>MTKPLDGINVLDFTHVAAGPACTQMMGFLGANVIKIERRGSGDMTRGWLQDKPNVDSLYFTMFNCNKRSIELDMKTPEGKELLEQMIKKADVMVENFGPGALDRMGFTWEYIQELNPRVILASVKGYAEGHANEHLKVYENVAQCSGGAAATTGFWDGPPTVSGAALGDSNSGMHLMIGILAALEIRHKTGRGQKVAVAMQDAVLNLVRIKLRDQQRLERTGILAEYPQAQPNFAFDRDGNPLSFDNITSVPRGGNAGGGGQPGWMLKCKGWETDADSYVYFTIAANMWPQICDMIDKPEWKDDPAYNTFEGRVDKLMDIFS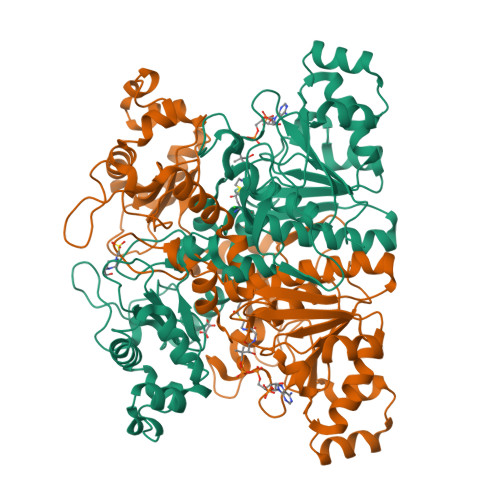FIETKFADKDKFEVTEWAAQYGIPCGPVMSMKELAHDPSLQKVGTVVEVVDEIRGNHLTVGAPFKFSGFQPEITRAPLLGEHTDEVLKELGLDDAKIKELHAKQVV[2x]>MRVIFSEDHKLRNAKTELYGGELVPPFEAPFRAEWILAAVKEAGFDDVVAPARHGLETVLKVHDAGYLNFLETAWDRWKAAGYKGEAIATSFPVRRTSPRIPTDIEGQIGYYCNAAETAISPGTWEAALSSMASAI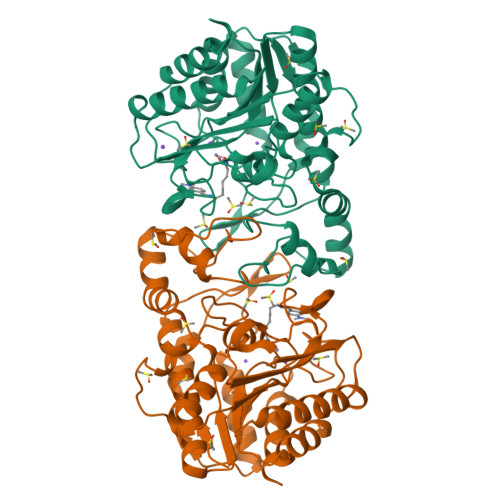DGADLIAAGHKAAFSLCRPPGHHAGIDMFGGYCFINNAAVAAQRLLDKGAKKIAILDVDFHHGNGTQDIFYERGDVFFASLHGDPAEAFPHFLGYAEETGKGAGAGTTANYPMGRGTPYSVWGEALTDSLKRIAAFGAEAIVVSLGVDTFEQDPISFFKLTSPDYITMGRTIAASGVPLLVVMEGGYGVPEIGLNVANVLKGVAG[12x]>[4x]MQNAGSLVVLGSINADHILNLQSFPTPGETVTGNHYQVAFGGKGANQAVAAGRSGANIAFIACTGDDSIGESVRQQLATDNIDITPVSVIKGESTGVALIFVNGEGENVIGIHAGANAALSPALVEAQRERIANASALLMQLESPLE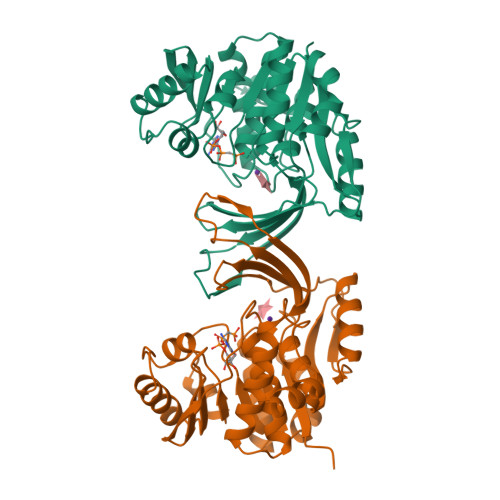SVMAAAKIAHQNKTIVALNPAPARELPDELLALVDIITPNETEAEKLTGIRVENDEDAAKAAQVLHEKGIRTVLITLGSRGVWASVNGEGQRVPGFRVQAVDTIAAGDTFNGALITALLEEKPLPEAIRFAHAAAAIAVTRKGAQPSVPWREEIDAFLDRQR>[2x]SSGNAKIGHPAPNFKATAVMPDGQFKDISLSDYKGKYVVFFFYPLDFTFVCPTEIIAFSDRAEEFKKLNSQVIGASVDSHFSHLAWVNT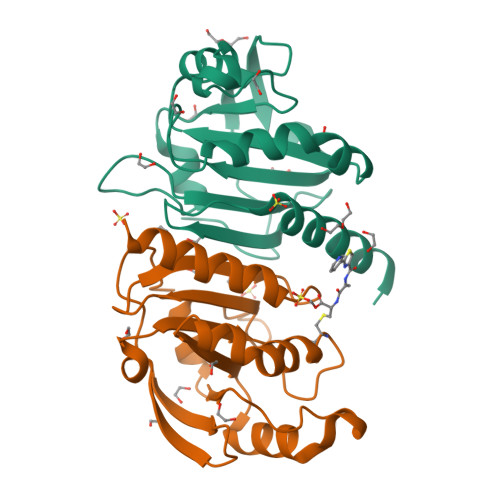PKKQGGLGPMNIPLVSDPKRTIAQDYGVLKADEGISFRGLFIIDDKGILRQITVNDLPVGRSVDETLRLVQAFQFTDKHGEVSPAGWKPGSDTIKPDVQKSKEYFSKQK>[2x]RRGSFVEMVDNLRGKSGQGYYVEMTVGSPPQTLNILVDTGSSNFAVGAAPHPFLHRYYQRQLSSTYRDLRKGVYVPYTQGKWEGELGTDLVSIPHGPNVTVR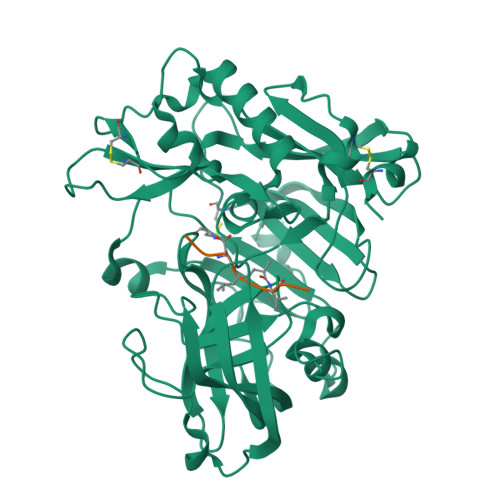ANIAAITESDKFFINGSNWEGILGLAYAEIARPDDSLEPFFDSLVKQTHVPNLFSLQLCGAGFPLNQSEVLASVGGSMIIGGIDHSLYTGSLWYTPIRREWYYEVIIVRVEINGQDLKMDCKEYNYDKSIVDSGTTNLRLPKKVFEAAVKSIKAASSTEKFPDGFWLGEQLVCWQAGTTPWNIFPVISLYLMGEVTNQSFRITILPQQYLRPVEDVATSQDDCYKFAISQSSTGTVMGAVIMEGFYVVFDRARKRIGFAVSACHVHDEFRTAAVEGPFVTLDMEDCGYN;>[2x]ELDXVEF> IRLPPEVNRILYIRNLPYKITAEEMYDIF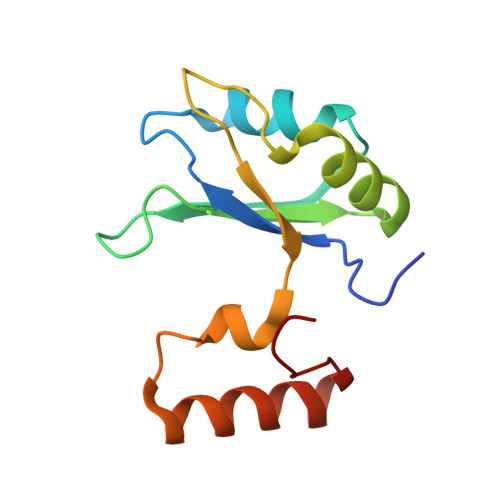GKYGPIRQIRVGNTPETRGTAYVVYEDIFDAKNAVDHLSGFNVSNRYLVVLYYNANRAFQKMDTKKKEEQLKLLKEKYGINTDPPK> GMSSKQHCVKLNDGHLIPALGFGTYKPKEVPKSKSLEAACLALDVGYRHVDTAYAYQVEEEIGQAIQSKIKAGVVKREDLFVTTKLWCTCFRPELVKPALEKSLKKLQLDYVDLYIMHYPVPMKSGDNDFPVNEQGKSLLDTVDFCDTWERLEECKDAGLVKSIGVSNFNHRQLERILNKPGLKYKPVCNQVECHLYLNQRKLLDYCESKDIVLVAYGALGTQRYKEWVDQNSPVLLNDPVLCDVAKKNKRSPALIALRYLIQRGIVPLAQSFKENEMRENLQVFGFQ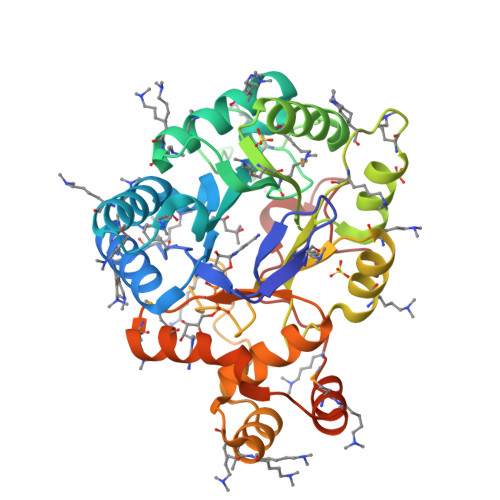LSPEDMKTLDGLNKNFRYLPAEFLVDHPEYPFVEEY> GPCH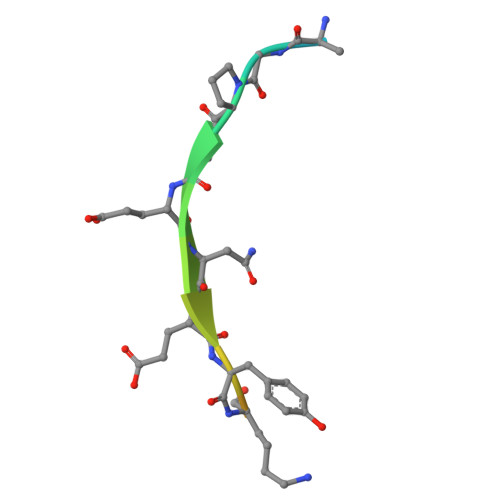GPEENEYKSEGTFGI> SPQPLEQIKLSESQLSGRVGMIEMDLASGRTLTAWRADERFPMMSTFKVVLCGAVLARVDAGDEQLERKIHYRQQDLVDYSPVSEKHLADGMTVGELCAAAIT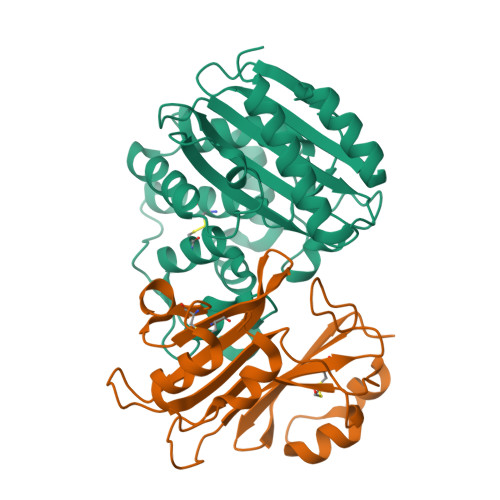MSDNSAANLLLATVGGPAGLTAFLRQIGDNVTRLDRWETELNEALPGDARDTTTPASMAATLRKLLTSQRLSARSQRQLLQWMVDDRVAGPLIRSVLPAGWFIADKTGAGERGARGIVALLGPNNKAERIVVIYLRDTPASMAERNQQIAGIGAALIEHWQR;> AGVMTGAKFTQIQFGMTRQQVLDIAGAENCETGGSFGDSIHCRGHAAGDYYAYATFGFTSAAADAKVDSKSQEKLLAPSAPTLTLAKFNQVTVGMTRAQVLATVGQGSCTTWSEYYPAYPSTAGVTLSLSCFDVDGYSSTGFYRGSAHLWFTDGVLQGKRQWDLV2'-deoxy-5-ethynyl-2',2'-difluorouridine | 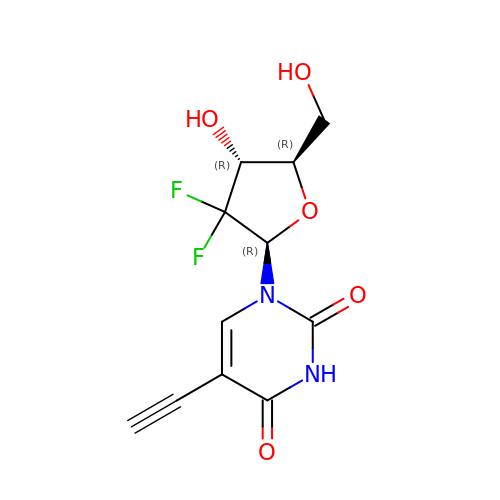C11 H10 F2 N2 O5 | JFVJRPYRLUHQTG-ZXFLCMHBSA-N> MAVTDLSLTNSSLMPTLNPMIQQLALAIAASWQSLPLKPYQLPEDLGYVEGRLEGEKLVIENRCYQTPQFRKMHLELAKVGKGLDILHCV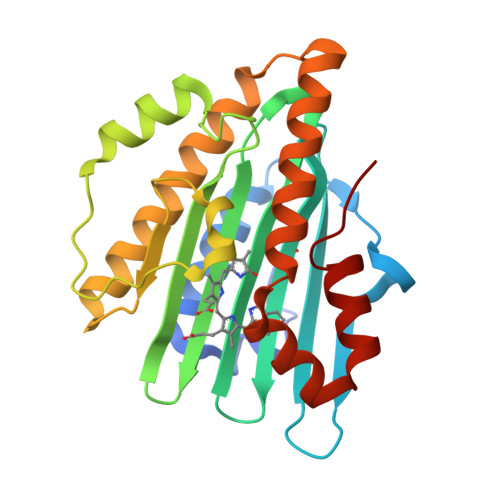MFPEPLYGLPLFGCDIVAGPGGVSAAIADLSPTQSDRQLPAAYQKSLAELGQPEFEQQRELPPWGEIFSEYCLFIRPSNVTEEERFVQRVVDFLQIHCHQSIVAEPLSEAQTLEHRQGQIHYCQQQQKNDKTRRVLEKAFGEAWAERYMSQVLFDVIQ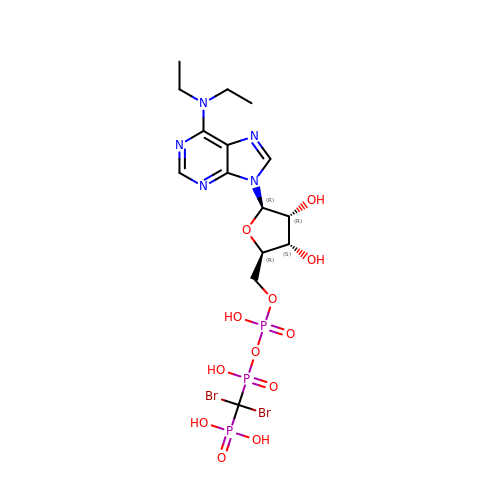5'-O-[(R)-{[(R)-[dibromo(phosphono)methyl](hydroxy)phosphoryl]oxy}(hydroxy)phosphoryl]-N,N-diethyladenosine | C15 H24 Br2 N5 O12 P3 | ILXFKEOLRYLPJG-IDTAVKCVSA-N The A. baumannii outer-membrane transporter protein, BauA, that recognises this siderophore has itself been identified as a vaccine candidate. The siderophore is known to be bound from the medium by the integral outer-membrane BauA protein. BauA has the typical outer-membrane TonB-dependent transporter (TBDT) fold with a β-barrel formed by 22 antiparallel strands, several extracellular loops, and a plug domain folded inside of the barrel. Acinetobactin is synthesized as a precursor, preacinetobactin, which rearranges non-enzymatically and irreversibly at pH >7 to give acinetobactin.

The apo structure of BauA was solved to a resolution of 1.8 Å by single wavelength anomalous diffraction (SAD) using selenomethionine-labeled proteins. Residues 33 to 703 of the protein are well defined in the electron density map, while the N-terminal region comprising the TonB box is missing, presumably because it is flexible. Compared to the other TBDTs, the extracellular loops of the β-barrel form a large open cavity bordered by mainly short and apolar amino acids giving large access to the loops NL1-NL3 of the plug domain. The asymmetric unit contains three monomers arranged around a threefold symmetry axis reminiscent of the porin arrangement and thus plausibly biologically meaningful. PISA, a computational assessment of oligomeric state in the crystal, suggests a trimer with a high degree of confidence. Biophysical methods (gel filtration and light scattering) do not support a trimeric assembly. Size Exclusion Chromatography coupled to Multi-Angle Light Scattering (SEC-MALS) analysis in C8E4 is consistent with monomer whilst native gel shows the protein runs more closely to a dimer; however, the detergent bound to the protein may increase the apparent weight suggesting a monomer in solution.

>[3x]GAMAVIDNSTKTLEQQTAQTNVAALPAITVKAEQDDTYAGGQVATSSNVGFLGSKKFLDTPFNTISYTDKYIEDKQAKDITEVIAATDPSIYTNGASGGWSENYYIRGYASSTNDMSMNGLFGITPFYRTSPEMFGRVEVLKGPSALLNGMPPAGSVGGTVNLVTKYAADEPFARLTTTYMSDAQFGGHVDVGRRFGENKEFGVRINGMYRDGDAAVNDQSKESRLFSLGLDWQGENARVFVDAYDALDHVDGVTRGVNVSTAVGIPKPPKADTLLSPDWGSVETKDKGAMIRGEYDFSDQLMAYAAYGQSTTEYKYNGASAGTITSSTGTLSSTLGQLAFDVDKKSADAGFKGKFETGSVKHQWVANATYYNHTQDDYGYRIIPGFSDPVITNIYDPNPNWGPKPEFTPPFLFHSTLSTSSFGLADTLSFAQDKVQLTLGLRHQTVKATSSVNTLPENAKSATTPGVALLIKATDKISVYANYIEGLTKGDQAPATASNPGEIFPPQKTKQQELGLKVDLGTFAHTLSAFEITKPSSYLDPSKLVNNLPTFVSDGEQRNRGIEWSFFGSPIEHVRLMGGFTYLDPELTKTKSGGNDGHTAVAVPKNQAKLGAEWDTQVAQGTLTLSGNINAVSKQYINAENTLSVPGRTLLDVGARYSTKVEDHPVTFRANIYNLTNKAYWAQPQLTNLALGAPRTYMLSVSYDF>[8x]SNADGRIFKMFIEHLEFEKGLDAFSQSWIKALEDSEFLAILRL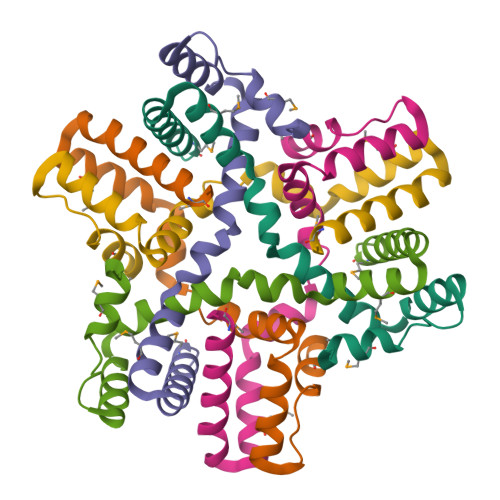LFHHIVTSESAHEFAANGIDRLYKMVESQFGSGGDKELEWLIGRSLIQMSK>GSHMTGELEVKNMDMKPGSTLKITGSIADGTDGFVINLGQGTDKLNLHFNPRFSESTIVCNSLDGSNWGQEQREDHLCFSPGSEVKFTVTFESDKFKVKLPDGHE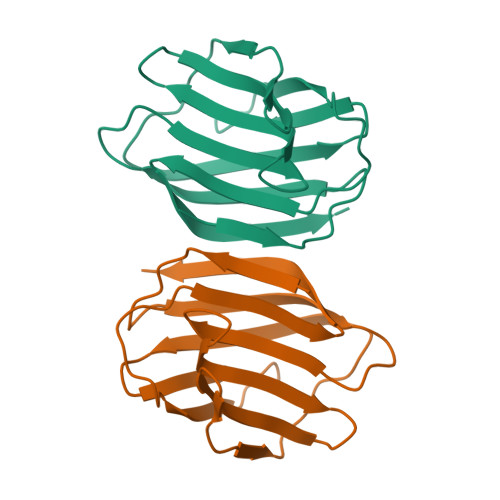LTFPNRLGHSHLSYLSVRGGFNMSSFKLKE[6x]1-[4-methyl-1-(methylsulfonyl)piperidin-4-yl]-1,6-dihydroimidazo[4,5-d]pyrrolo[2,3-b]pyridine 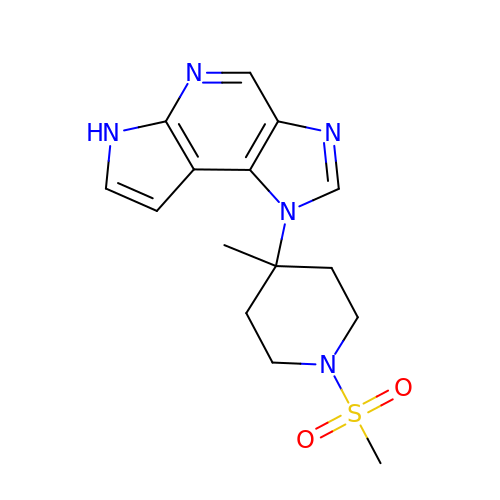| C15 H19 N5 O2 S | NWNODCMQDYQNDW-UHFFFAOYSA-N>[2x]XTYSITLRVFQRNPGRGFFSI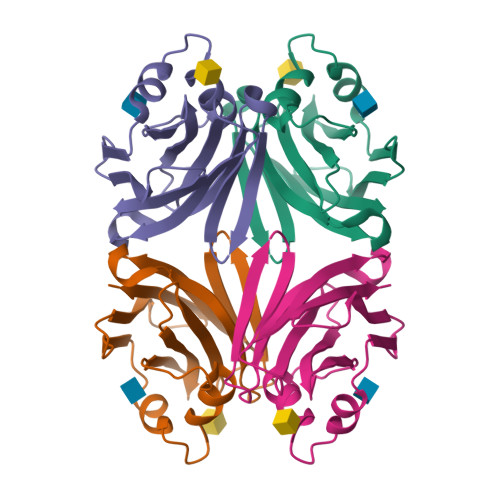VEKTVFHYANGGTWSEAKGTHTLTMGGSGTSGVLRFMSDKGELITVAVGVHNYKRWCDVVTGLKPEETALVINPQYYNNGPRAYTREKQLAEYNVTSVVGTRFEVKYTVVEGNNLEANVIFS> GGAXAUA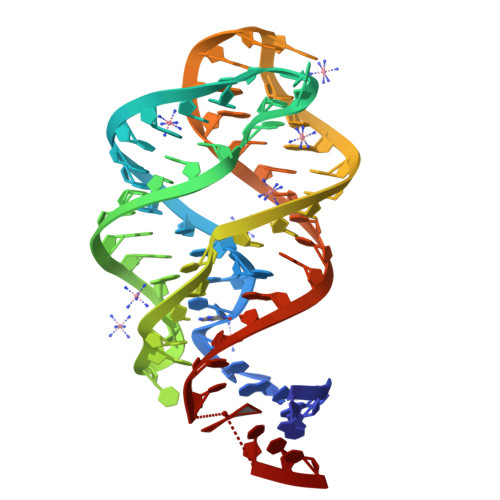UAAUCGCGUGGAUAUGGCACGCAAGUUUCUACCGGGCACCGUAAAUGUCCGACUAUXUCC>[5x]MSEKNVSIVVAASVLSSGIGINGQLPWSISEDLKFFSKITNNKCDSNKKNALIMGRKTWDSIGRRPLKNRIIVVISSSLPQDEADPNVVVFRNLEDSIENLMNDDSIENIFVCGGESIYRDAL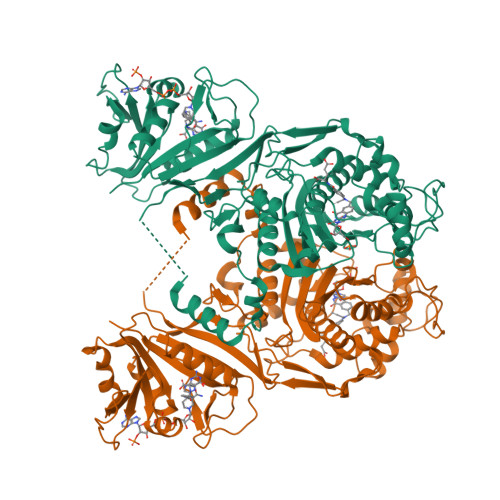KDNFVDRIYLTRVALEDIEFDTYFPEIPETFLPVYMSQTFCTKNISYDFMIFEKQEKKTLQNCDPARGQLKSIDDTVDLLGEIFGIRKMGNRHKFPKEEIYNTPSIRFGREHYEFQYLDLLSRVLENGAYRENRTGISTYSIFGQMMRFDMRESFPLLTTKKVFIRGIFEELIWFIKGDTNGNHLIEKKVYIWSGNGSKEYLERIGLGHREENDLGPIYGFQWRHYNGEYKTMHDDYTGVGVDQLAKLIETLKNNPKDRRHILTAWNPSALSQMALPPCHVLSQYYVTNDNCLSCNLYQRSCDLGLGSPFNIASYAILTMMLAQVCGYEPGELAIFIGDAHIYENHLTQLKEQLSRTPRPFPQLKFKRKVENIEDFKWEDIELIGYYPYPTIKMDMAV> MGSSHHHHHHHHHHSSGLVPRGSHIDPPVIDAGAVPPDETGPDQPTEQRKICATPTVMPNSNFADRPWANDYLRIQEAQKFATGAGVTVAVIDTG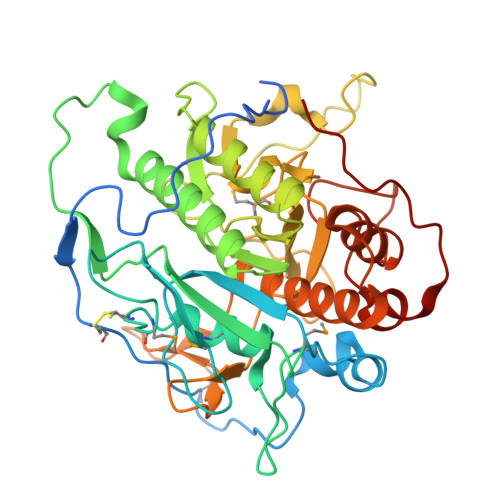VNGSPRVPAEPGGDFVDAAGNGMSDCDAHGTMTAAIIGGRPSPTDGFVGMAPDVRLLSLRQTSVAFQPKGARQDPNDPNTTQTAGSIRSLARSVVHAANLGAQVINISEAACYKVTRRIDETSLGAAINYAVNVKGAVIVVAAGNTGQDCSQNPPPAPSVPSDPRGWREVQTIVSPAWYAPLVLTVGSIGQNGQPSNFSMSGPWVGAAAPGENLTSLGYDGQPVNATPGEDGPVPLNGTSFSAAYVSGLAALVKQRFPDLTPAQIINRITATARHPGGGVDNYVGAGVIDPVAALTWEIPDGPEKAPFRVKEV>MWFGEFGGQYVPETLVGPLKELEKAYKRFKDDEEFNRQLNYYLKTWAGRPTPLYYAKRLTEKIGGAKVYLKREDLVHGGAHKTNNAIGQALLAKLMGKTRLIAETGAGQHGVATAMAGALLGMKVDIYMGAEDVERQKMNVFRMKLLGANVIPVNSGSRTLKDAINEALRDWVATFEYTHYLIGSVVGPHPYPTIVRDFQSVIGREAKAQILEAEGQLPDVIVACVGGGSNAMGIFYPFVNDKKVKLVGVEAGGKGLESGKHSAS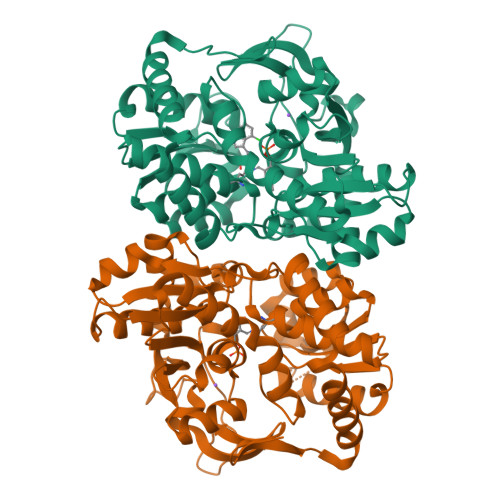LNAGQVGVSEGMLSYFLQDEEGQIKPSHSIAPGLDYPGVGPEHAYLKKIQRAEYVAVTDEEALKAFHELSRTEGIIPALESAHAVAYAMKLAKEMSRDEIIIVNLSGRGDKDLDIVLKASGNVLEHHHHHH[4x]>[2x]MNQSASEQLQTDIPASISAMVLLNSACQGVVETYIDQGNAEHWYAQVEQNLNAVQKLVRQWRLSGNLYFSNDIMDSVLSIANTFKDSNVQILT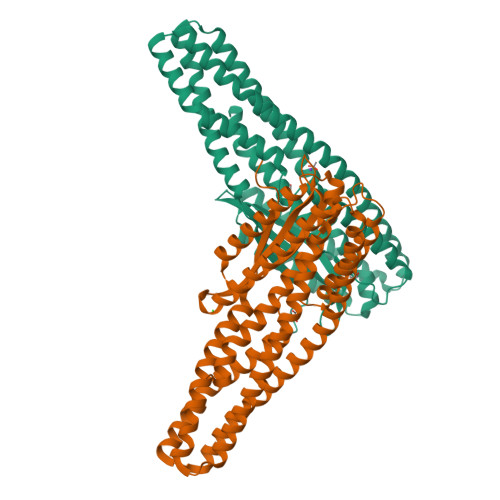LFKALETRFDTAQLQQLTSLILTLQNPIQSLTSNIKRYDEGLNAWARQVEDAHNTLQQTIAQIQQEEVSIQAEIIATNAQIDLMKQQIAAFKTAIANAQSQRKKGIFETIFGVVLAPFTLGGSLILAGFGVSSIVEAQSEISSLQSDIQSSLNTINHDQQTLSQDQQQIASLNALLLSVDQVNNDCAAISRSLDTLQTTVLSLYNETNNVVSNLTKAQDSQAVILEQVWYQSAYNEWQDILEVASTLNNAQPQITKAQIKENLYFE>GSHMATFLIKHKASGKFLHPKGGSSNPANDTNLVLHSDIHERMYFQFDVVDERWGYIKHAASGKIVHPLGGKADPPNETKLVLHQDRHDRALFAMDFFNDNIIHKAGKYVHPKGGSTNPPNETLTVMHGDKHGAMEFI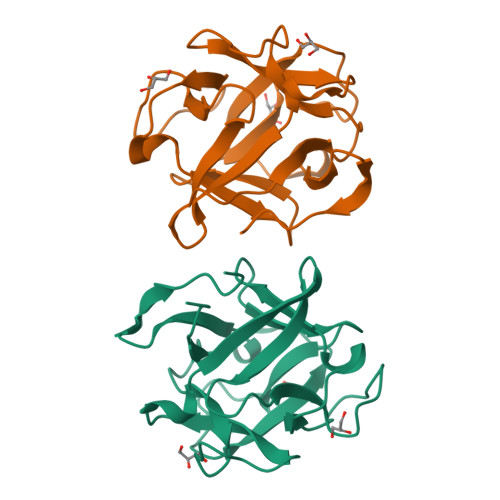FVSPKNKDKRVLVYV[2x]> MMSESLSLPKDFEWGFATAAYQIEGAVKEGGRGPSIWDTYCHLEPSRTNGANGDVACDHYHRYDEDFDLLTKYGAKAYRFSLSWSRIIPLGGRLDPINEEGIQFYSNLI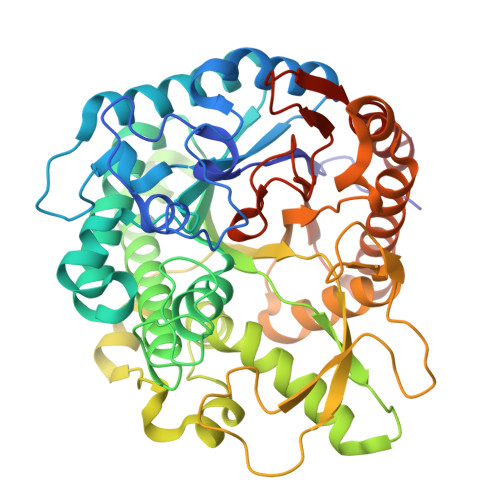DALLKRGVTPWVTLYHWDLPQALHDRYGGWLNVKEVQLDFERYARLCFERFGDRVKNWITINEPWIQSIYGYATGSNAPGRSSINKHSTEGDTTTEPWLAGKAQIMSHARAVAVYSKDFRASQKGQIGISLNGDYYEPWDSSDPRDKEAAERRMEFHIGWYANPIFLKKDYPASMRKQLGDRLPALTPADFAILNAGETDFYGMNYYTSQFARHYEGPVPKTDFLGAIHEHQENKDGSPVGEESGIFWLRSCPDMFRKHLARVHGLYGKPIYITENGCPCPGEDKMTCEEAINDPFRIQYFDSHLDSISKAISQDGVVVKGYFAWALLDNLEWSDGYGPRFGVTYTDYTTLKRTPKKSALVLKDMFADRQRVKVAA> MTTPSHLSDRYELGEILGFGGMSEVHLARDLRLHRDVAVKVLRADLARDPSFYLRFRREAQNAAALNHPAIVAVYDTGEAETPAGPLPYIVMEYVDGVTLRD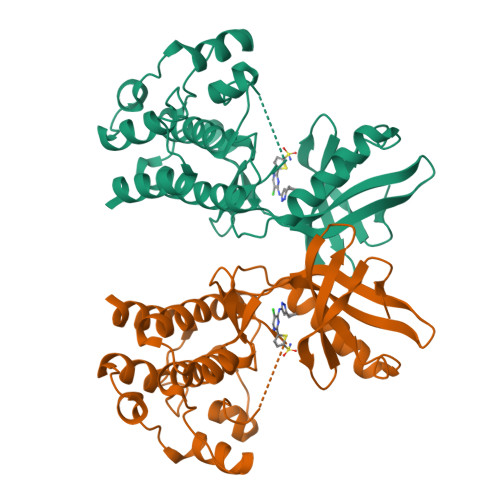IVHTEGPMTPKRAIEVIADACQALNFSHQNGIIHRDVKPANIMISATNAVKVMDFGIARAIADSGNSVTQTAAVIGTAQYLSPEQARGDSVDARSDVYSLGCVLYEVLTGEPPFTGDSPVSVAYQHVREDPIPPSARHEGLSADLDAVVLKALAKNPENRYQTAAEMRADLVRVHNG>[2x]GSHMDSTTIQQNK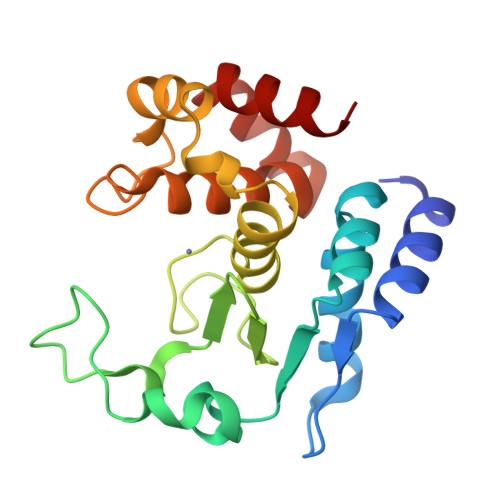DTLSQIVVFPTGNYDKNEANAMVNRLANIDGKYLNALKQNNLKIKLLSGKLTDEKEYAYLKGVVPKGWEGTGKTWDDVPGLGGSTVALRIGFSNKGKGHDAINLELHETAHAIDHIVLNDISKSAQFKQIFAKEGRSLGNVNYLGVYPEEFFAESFAYYYLNQDTNSKLKSACPQTYSFLQNLAK>MLEEYRKHVAERAAEGIAPKPLDANQMAALVELLKNPPAGEEEFLLDLLTNRVPPGVDEAAYVKAGFLAAIAKGEAKSPLLTPEKAIELLGTMQGGYNIHPLIDALDDAKLAPIAAKALSHTLLMFDNFYDVEEKAKAGNEYAKQVMQSWADAEWFLNRPALAEKLTVTVFKVTGETNTDDLSPAPDAWSRPDIPLHALAMLKNAREGIEPDQPGVVGPIKQIEALQQKGFPLAYVGDVVGTGSSRKSATNSVLWFMGDDIPHVPNKRGGGLCLGGKIAPIFFNTMEDAGALPIEVDVSNLNMGDV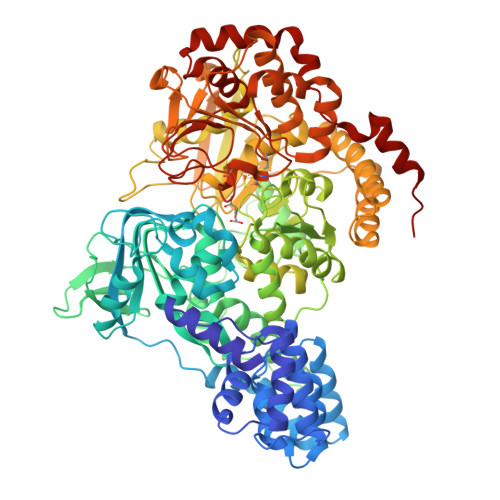IDVYPYKGEVRNHETGELLATFELKTDVLIDEVRAGGRIPLIIGRGLTTKAREALGLPHSDVFRQAKDVAESDRGFSLAQKMVGRACGVKGIRPGAYCEPKMTSVGSQDTTGPMTRDELKDLACLGFSADLVMQSFCHTAAYPKPVDVNTHHTLPDFIMNRGGVSLRPGDGVIHSWLNRMLLPDTVGTGGDSHTRFPIGISFPAGSGLVAFAAATGVMPLDMPESVLVRFKGKMQPGITLRDLVHAIPLYAIKQGLLTVEKKGKKNIFSGRILEIEGLPDLKVEQAFELTDASAERSAAGCTIKLNKEPIIEYLNSNIVLLKWMIAEGYGDRRTLERRIQGMEKWLANPELLEADADAEYAAVIDIDLADIKEPILCAPNDPDDARPLSAVQGEKIDEVFIGSCMTNIGHFRAAGKLLDAHKGQLPTRLWVAPPTRMDAAQLTEEGYYSVFGKSGARIEIPGCSLCMGNQARVADGATVVSTSTRNFPNRLGTGANVFLASAELAAVAALIGKLPTPEEYQTYVAQVDKTAVDTYRYLNFNQLSQYTEKADGVIFQTAV[2x]> SSLENVVYNLVNAGHFDGRAGELPCAVIGEKVIAKIQNEDVVVFKNNTPFPTNVAVELFAKRSIRPHPELKLFRNLNIDVCWSHVLWDYAKDSVFCSSTYKVCKYTDLQCIESLNVLFDGRDNGALEAFKKCRNGVYINTTKIKSLSMIKGPQRADLNGVVVEKVGDSDVEFWFAVRKDGDDVIFSRTGSLEPSHYRSPQGNPGGNRVGDLSGNEALARGTIFTQSRLLSSFTPRSEMEKDFMDLDDDVFIAKYSLQDYAFEHVVYGSFNQKIIGGLHLLIGLARRQQKSNLV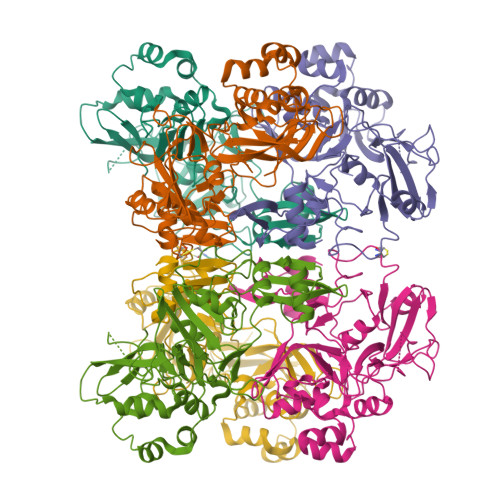IQEFVTYDSSIHSYFITDENSGSSKSVCTVIDLLLDDFVDIVKSLNLKCVSKVVNVNVDFKDFQFMLWCNEEKVMTF>MKEVTIEIKNKTGLHARPAALFVQTASKFSSQIWVEKDNKKVNAKSIMGIMSLGVSQGNVVKLSAEGDDEEEAIKALVDLIESKFGEELEHHHHHH[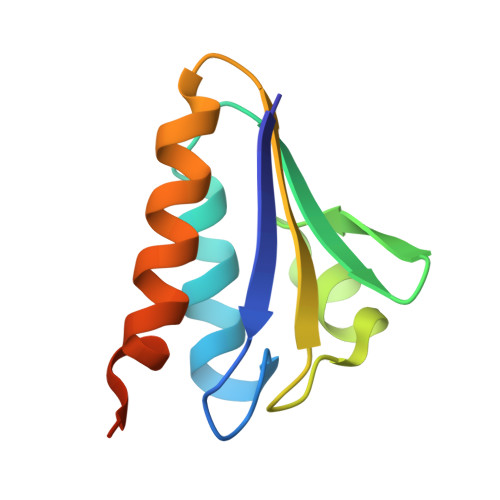3x]> XIWLLQELLRL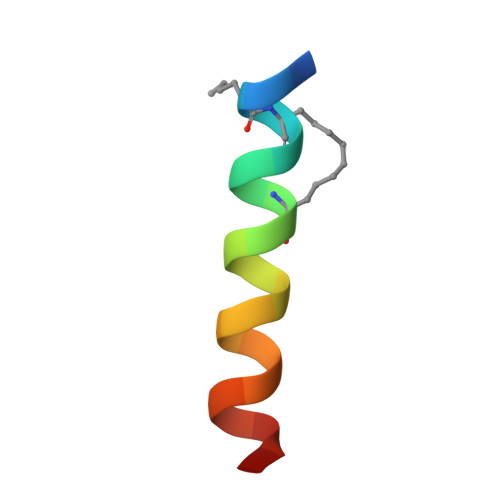GDEINARYARX>GSHMATYYYALASQKFLLEEEPFEEVLKERRRDYGEKNKEIDFWQVIQPAFLNAPELAEAKAKAPEKNVAIVSTNKSFIVWVKLALEYVLTGEFEAPSDAIPDPLASLD[4x]

Mg-protoporphyrin IX monomethylester cyclase (MgPME–cyclase) catalyses the formation of the isocyclic E ring by cyclising the methyl propionate side-chain at C-13 to the C-15 bridge carbon between rings C and D, generating protochlorophyllide (Pchlide). Recently, the small monomeric protein Ycf54 was identified as a second candidate component of the MgPME–cyclase. The Ycf54 protein has been identified as a component of the MgPME–cyclase complex.

To investigate the structural basis for these effects of the A9G and R82A mutations in Synechocystis, crystal structures solved by molecular replacement against the WT Synechocystis Ycf54 were obtained for these two proteins to resolutions of 1.5 Å and 2.2 Å, respectively. Superposition of the A9G and R82A models on WT Ycf54 resulted in respective RMSDs of 0.19 Å and 0.28 Å over all Cα atoms, showing that there are no significant structural alterations between the WT and mutant structures. Upon closer inspection of the R82A structure, differences are observed in both the local hydrogen bonding network and surface electrostatics. In WT Ycf54, R82 adopts two clearly defined conformations, both of which form stabilising hydrogen bonds with neighbouring residues. In one conformation, R82 forms a water-mediated hydrogen bond with the side chain of W78, and in the other R82 forms two direct hydrogen bonds with the backbone carbonyl of F20 and the side chain of E17. All of these interactions are lost in R82A, which may alter the stability of this region. Examination of the surface electrostatics shows the base substitution to alanine changes the surface electrostatics from predominantly positive in WT Ycf54 to predominantly negative in R82A. It may be that the flexibility of R82, along with its associated positive surface potential, is required for docking of Ycf54 onto CycI and consequently mediation of the cyclase reaction. The structure of Ycf54.R82A, which has impaired Chl biosynthesis, ∼50% reduction in CycI levels and abolished interaction with CycI, reveals that the R82A mutation has reversed the normally positive surface electrostatics to yield an overall negative face. The rest of the R82A Ycf54 structure remains unaltered by the arginine to alanine substitution; therefore, it is reasonable to conclude that this residue is required for Ycf54 to form a stable interaction with CycI.3-bromanyl-1~{H}-indazole-5-carboxylic 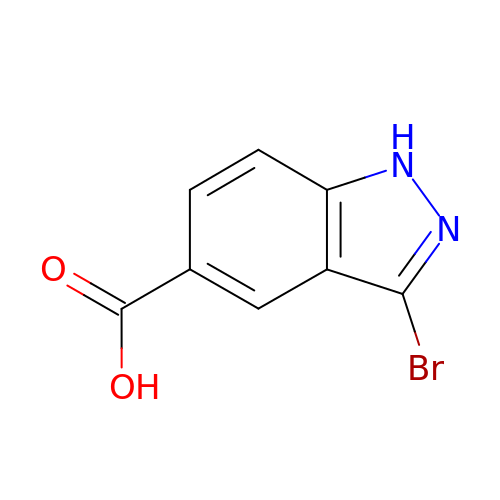acid | C8 H5 Br N2 O2 | RWQMEUDBXGKAER-UHFFFAOYSA-N The archetypal cofactor-free oxidase is uricase (urate oxidase or rasburicase, UOX), a long-investigated, therapeutically important (commercialized as Elitek in the US and Fasturtec in Europe), tetrameric 133 kDa enzyme that catalyzes the O2-mediated degradation of uric acid (UA) to 5-hydroxyisourate (5-HIU). A number of oxidases and oxygenases, however, operate in a cofactor-free manner, relying on very limited chemical tools to promote and control O2 chemistry. X-ray crystallography at near-atomic resolution together with in crystallo Raman spectroscopy and QM/MM methods offer unambiguous evidence for a C5-peroxide intermediate in cofactor-free UOX catalysis.

To investigate the reaction steps involving dioxygen in UOX-mediated catalysis, we employed 9-methyl uric acid (MUA) as we reasoned that methyl substitution at position 9 could stabilize the putative peroxide intermediate. Crystallographic analysis at near-atomic resolution (see Table S1 for data collection and refinement statistics) showed that under strict anaerobic conditions, MUA binds, as do UA and several inhibitors,[2a, 7] at the interface between two UOX protomers in a 35 Å3 cavity exposed to the solvent on the side of the substrate’s imidazole ring. A combination of hydrogen bonds, salt bridges, and hydrophobic interactions holds the flat MUA in place. A water molecule (W1) is held above the C4=C5 bond at a distance of 3.0 Å from the MUA plane by H-bonds with T57(Oγ1) and N254(Nδ2). An additional water molecule (W2), part of a complex solvent network, interacts with the O8 atom of the substrate. In order to define the vibrational modes responsible for the observed changes, we employed QM/MM methods at the MP2/6-31+G* level of theory. Calculations carried out for the organic species in their protein environment predict a band at 600 cm−1 (experimental 605 cm−1) for the 5-PMUA hydroperoxide (brown trace in Figure 3 c) and a band at 597 cm−1 (experimental 597 cm−1) for the MUA dianion (green). Ring distortions account for the MUA 597 cm−1 band.

> SAVKAARYGKDNVRVYKVHKDEKTGVQTVYEMTVCVLLEGEIETSYTKADNSVIVATDSIKNTIYITAKQNPVTPPELFGSILGTHFIEKYNHIHAAHVNIVCHRWTRMDIDGKPHPHSFIRDSEEKRNVQVDVVEGKGIDIKSSLSGLTVLKSTNSQFWGFLRDEYTTLKETWDRILSTDVDATWQWKNFSGLQEVRSHVPKFDATWATAREVTLKTFAEDNSASVQATMYKMAEQILARQQLIETVEYSLPNKHYFEIDLSWHKGLQNTGKNAEVFAPQSDPNGLIKCTVGRSSLKSKL>AYTTFSQTKNDQLKEPMFFGQPVNVARYDQQKYDIFEKLIEKQLSFFWRPEEVDVSRDRIDYQALPEHEKHIFISNLKYQTLLDSIQGRSPNVALLPLISIPELETWVETWAFSETIHSRSYTHIIRNIVNDPSVVFDDIVTNEQIQKRAEGISSYYDELIEMTSYWHLLGEGTHTVNGKTVTVSLRELKKKLYLCLMSVNALEAIRFYVSFACSFAFAERELMEGNAKIIRLIARDEALHLTGTQHMLNLLRSGADDPEMAEIAEECKQECYDLFVQAAQQEKDWADYLFRDGSMIGLNKDILCQYVEYITNIRMQAVGLDLPFNTRSNPIPWINTWLVSDNVQVA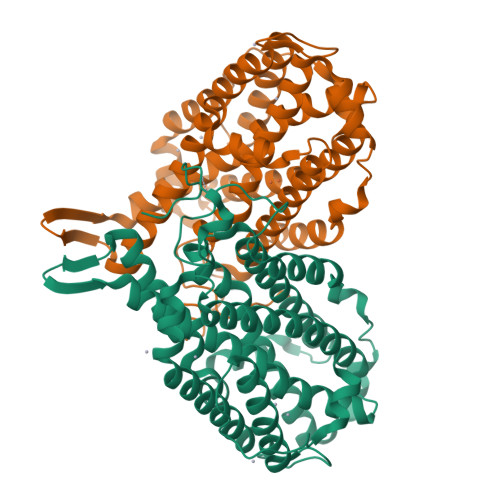PQEVEVSSYLVGQIDSEVDTDDLSNFQL[2x]>[3x]MGSSHHHHHHS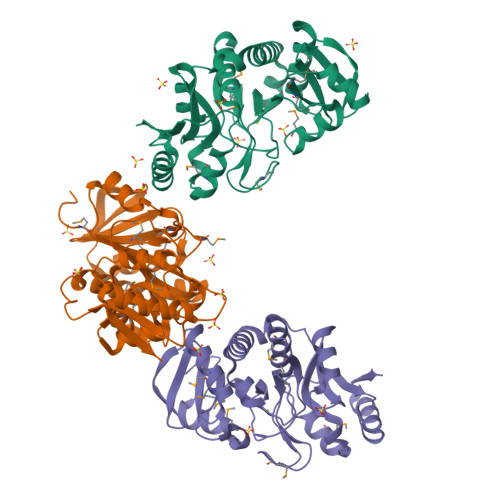SGRENLYFQGHMKVIMTTKVDKASMNIMNKLIENFGFKETEYVFEGNPVYKRGDVLILTTNDEMIYYDYLDREIENQLGFKPEIIAFASRHSSKQKLPALTTHVTGNWGKAMYGGKDESFAVAIPSAMKLSLLKMSELNDLGWTVCYEATHHGPTELEVPSFFIEIGSSEEEWINDRAGEIIAETIIYVLDNYEKGRSKFKVALGIGGGHYAPKQTKRALEGDLAFGHILPKYAQPVSRDVMIKALNRFGEKVEAIYVDWKGSRGETRQLAKSLAQELGLEFIKDGS> SGISLDNSYKMDYPEMGLCIIINNKNFHKSTGMTSRS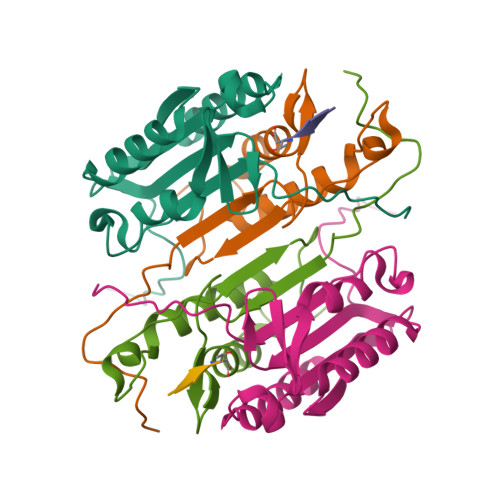GTDVDAANLRETFRNLKYEVRNKNDLTREEIVELMRDVSKEDHSKRSSFVCVLLSHGEEGIIFGTNGPVDLKKITNFFRGDRCRSLTGKPKLFIIQACRGTELDCGIET;> ASGVDDDMACHKIPVEADFLYAYSTAPGYYSWRNSKDGSWFIQSLCAMLKQYADKLEFMHILTRVNRKVATEFESFSFDATFHAKKQIPCIVSMLTKELYFYH>[6x]MHHHHHHQHQHENLYFQGMQTKKNEIWVGIFLLAALLAALFVCLKAANVTSIRTEPTYTLYATFDNIGGLKARSPVSIGGVVVGRVADITLDPKTYLPRVTLEIEQRYNHIPDTSSLSIRTSGLLGEQYLALNVGFEDPELGTAILKDGDTIQDTKSAMVLEDLIGQFLYGSKGDDNKNSGDAPAAAPGNNETTEPVGTTK;>[2x]MLLNALASLGHKGIKTLRTFGRAGLMLFNALVGKPEFRKHAPLLVRQLYNVGVLSMLIIVVSGVFIGMVLGLQGYLVLTTYSAETSLGMLVALSLLRELGPVVAALLFAGRAGSALTAEIGLMRATEQLSSMEMMAVDPLRRVISPRFWAGVISLPLLTVIFVAVGIWGGSLVGVSWKGIDSGFFWSAMQNAVDWRMDLVNCLIKSVVFAITVTWISLFNGYDAIPTSAGISRATTRTVVHSSLAVLGLDFVLTALMFGN;>MEQSVANLVDMRDVSFTRGNRCIFDNISLTVPRGKITAIMGPSGIGKTTLLRLIGGQIAPDHGEILFDGENIPAMSRSRLYTVRKRMSMLFQSGALFTDMNVFDNVAYPLREHTQLPAPLLHSTVMMKLEAVGLRGAAKLMPSELSGGMARRAALARAIALEPDLIMFDEPFVGQDPITMGVLVKLISELNSALGVTCVVVSHDVPEVLSIADHAWILADKKIVAHGSAQALQANPDPRVRQFLDGIADGPVPFRYPAGDYHADLLPGS[2x];>MSESLSWMQTGDTLALSGELDQDVLLPLWEMREEAVKGITCIDLSRVSRVDTGGLALLLHLIDLAKKQGNNVTLQGVNDKVYTLAKLYNLPADVLPR[2x]

The Mla system, an ABC transporter in E. coli and related Gram-negative bacteria, has recently emerged as a key player in phospholipid transport across the bacterial envelope. Mla trafficks phospholipids between the IM and OM and is important for maintaining the outer membrane barrier. The IM complex, MlaFEDB, consists of four different proteins: MlaD, a membrane anchored protein from the MCE (Mammalian Cell Entry) protein family, which forms a homohexameric ring in the periplasm; MlaE (also called YrbE), a predicted integral inner membrane ABC permease; MlaF, an ABC ATPase; and MlaB, a STAS (Sulfate Transporter and Anti-Sigma factor antagonist) domain protein with possible regulatory function. The MlaFEDB transporter is significantly larger and more complicated than most other structurally characterized ABC transporters, consisting of a total of 12 polypeptide chains from four different genes, with a stoichiometry of MlaF2E2D6B2.

In addition, we resolved both coils of the membrane scaffold protein (MSP) belt surrounding the nanodisc using the map filtered at 6 Å, thereby clearly defining the position of the transmembrane domain. Our cryo-EM structure reveals that the core TMD of MlaE consists of five transmembrane helices (TM1 - TM5). While the vast majority of ABC transporter structures adopt an inward-open conformation in the absence of nucleotide, our structure of MlaE is in the outward-open state. Indeed, in our structure of the MlaFEDB complex, the pore of MlaD and the outward-open pocket of MlaE line up with each other, resulting in a continuous hydrophobic pathway that runs from the pocket of MlaE, through MlaD, and out into the periplasm. Additional density was apparent in the outward-open pocket of MlaE, which is the right size and shape to accommodate two diacyl phospholipids. We modeled these as the most abundant PL species in E. coli, phosphatidylethanolamine, and these lipids make extensive contacts with both MlaE subunits, as well as MlaD. Strikingly, the second lipid (lipid 2) adopts an extended conformation, with one acyl chain reaching down into the MlaE pocket, while the other projects upwards to insert into a constriction in the MlaD pore formed by Leu106 and Leu107, which have previously been implicated in MlaD function. Thus, the asymmetry in MlaD appears to arise from its asymmetric interactions with lipid 1 at the interface of MlaE and MlaD.>[3x]MPLGLLWLGLALLGALHAQAQDSTS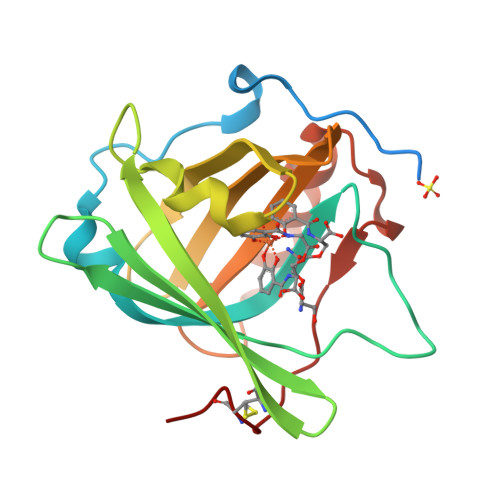DLIPAPPLSKVPLQQNFQDNQFQGKWYVVGLAGNAILREDKDPQKMYATIYELKEDKSYNVTSVLFRKKKCDYWIRTFVPGSQPGEFTLGNIKSYPGLTSYLVRVVSTNYNQHAMVFFKKVSQNREYFAITLYGRTKELTSELKENFIRFSKSLGLPENHIVFPVPIDQCIDG> GSHMS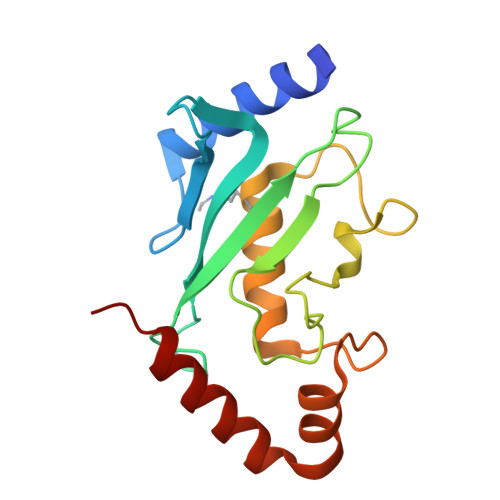GIALSRLAQERKAWRKDHPFGFVAVPTKNPDGTMNLMNWECAIPGKKGTPWEGGLFKLRMLFKDDYPSSPPKCKFEPPLFHPNVYPSGTVCLSILEEDKDWRPAITIKQILLGIQELLNEPNIQDPAQAEAYTIYCQNRVEYEKRVRAQAKKFAPS>CCAAGCTTGG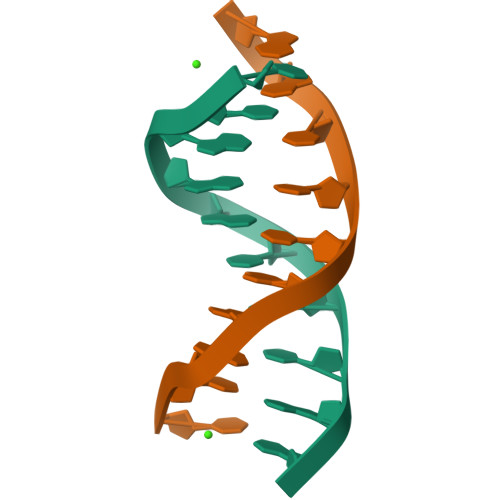[2x]>[6x]MDYKLKADEYNVTKAILSSAFKMWMDVIEVDVAIVGGGPSGLTAGKYLAKEGLKVVILERHLSFGGGTWGGGMGFPYIVVEE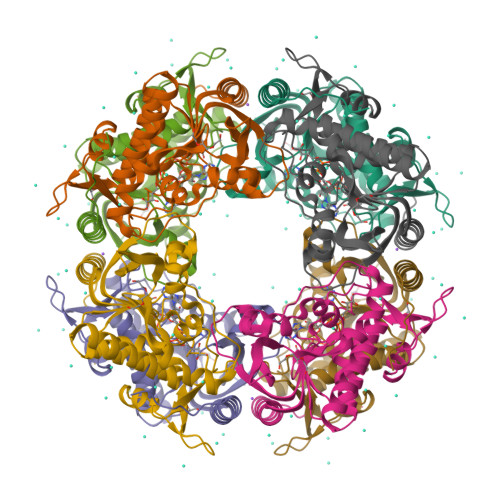PADEILRDAGIKLEKVEDVEGYYIADSVEVPAKLGASAIDAGAKILTSVAVEDLILREDKVAGVVVQGYAIEKAGLHVDPITINAKYVIDATGHDASVTTTLARKNKDLGIEVPGEKSMWADKGENSLLRNTREVYPGLFVCGMAANAVHAGYRMGAIFGGMYLSGKKCAEMILEKLNK>[2x]ADFEVHMLNKGKD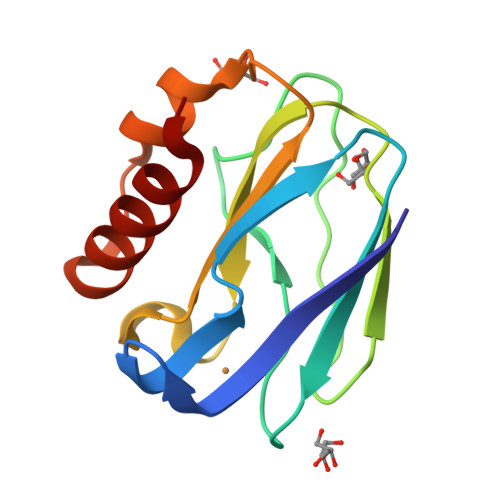GAFVFEPASLKVAPGDTVTFIPTDKGHNVETIKGMIPDGAEAFKSKINENYKVTFTAPGVYGVKCTPHYGMGMVGVVQVGDAPANLEAVKGAKNPKKAQERLDAALAALGN> AAGCAGACCTGACTGCACTCA;> AGTCA;> TCTGAGTGC;> GGTCTGC

In this work, we exhaustively probe the ability of all 36 immobile HJ sequences to form DNA crystals in two different designed systems. Three separate self-assembling DNA crystal systems are described in this report: the “4 × 5” and “4 × 6” designs (collectively referred to as the 4 × N systems), and a third construct with a “scrambled” sequence variant of the 4 × 6 lattices. Self-assembly was mediated by three constituent oligonucleotides: (S1) containing four sequence repeats of either 5 or 6 bases; (S2) composed of 21 bases containing complementary regions to both (S1); and (S3) which forms the second junction crossover. The HJ serves as the fundamental component at the core of each unit, and the ultimate assembly of the full lattice is facilitated by the complementary 2-base sticky ends that tail each duplex.

The 4 × 5 system robustly crystallized with 75% of the junctions, and we obtained crystals in all but 9 of 36 sequences. Pos1 and 2 were readily observable in the electron density maps at either one or both of these conserved sites in a significant number of the structures, with no apparent respect to motif or symmetry. Stereoscopic view, using J21 in the 4 × 5 system, 2Fo–Fc electron density accounting for the bases at the crossover regions are contoured at σ = 2.0, and the individual ion positions 1 and 2 (indicated Pos1 and Pos2) are independently contoured in the corresponding electron density at σ = 4.0. The presence of arsenic at these sites was substantiated by transferring the crystals into TAE-Mg2+ (40 mM Tris, 20 mM acetate, and 1 mM EDTA pH = 8.6), and subsequently freezing the crystals. The crystals were scanned at the arsenic K edge (λ = 1.04 Å) where the corresponding arsenate peak was present. No other components within the crystallization buffers could account for the resulting peaks in the Fo–Fc difference maps for the ions at their corresponding sites. However, in the majority of the crystal structures reported here, the cacodylate anion indeed fits best into the electron density map of our X-ray structures, due to the presence of sodium cacodylate in the crystallization solution.> GPAMRIISVNVNGIQAAAERGLLSWLQAQNADVICLQDTRASAFDLDDPSFQLDGYFLYACDAELPEQGGVALYSRLQPKAVISGLGFETADRYGRYLQADFDKVSIATLLLPSGQSGDESLNQKFKFMDDFTHYLSKQRRKRREYIYCGSLYVAHQKMDVKNWRECQQMPGFLAPERAWLDEVFGNLGYADALREVSREGDQFSWWPDSEQAEMLNLGWRFDYQVLTPGLRRFVR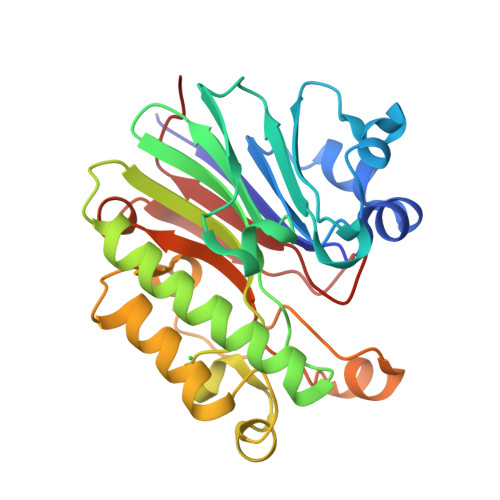NAKLPRQPRFSQHAPLIVDYDWQLSI N-acetyl-L-tyrosine | C11 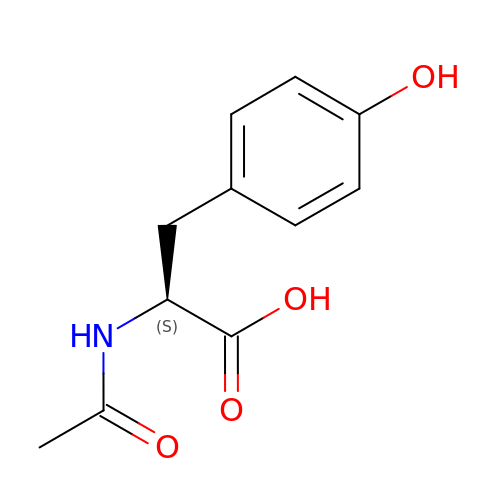H13 N O4 | CAHKINHBCWCHCF-JTQLQIEISA-N> SLRFLFEGQR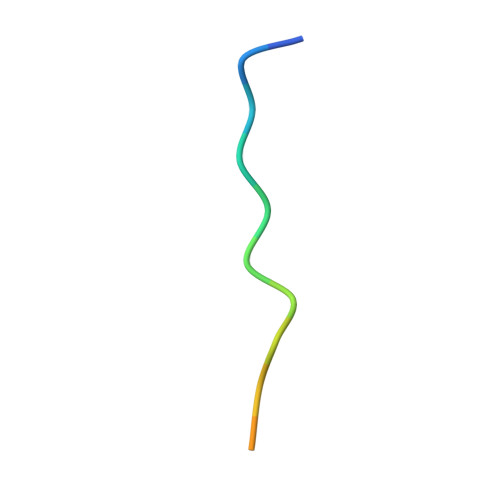IADNH> MAVDSAMELLFLDTFKHPSAEQSSHIDVVRFPCVVYINEVRVIPPGVRAHSSLPDNRAYGETSPHTFQLDLFFNNVSKPSAPVFDRLGSLEYDENTSIIFRPNSKVNTDGLVLRGWYNCLTLAIYGSVDRVISHDRDSPPPPPPPPPPPQPQPSLKRNPKHADGEKEDQFNGSPPRPQPRGPRTPPGPPPPDDDEDDPVPLPVSGDKEEDAPHREDYFEPISPDRNSVPQEGQYSDEGEVEEEQQEEGEEDEDDVDVEEEEDEDEDDRRTVDSIPEEEEEDEEEEGEEDEEGEGDDGYEQISSDEDGIADLERETFKYPNFDVEYTAEDLASVPPMTYDPYDRELVPLLYFSCPYKTTFEIEISRMKDQGPDKENSGAIEASVKLTELLDLYREDRGAKWVTALEEIPSLIIKGLSYLQLKNTKQDSLGQLVDWTMQALNLQVALRQPIALNVRQLKAGTKLVSSLAECGAQGVTGLLQAGVISGLFELLFADHVSSSLKLNAFKALDSVISMTEGMEAFLRGRQNEKSGYQKLLELILLDQTVRVVTAGSAILQKCHFYEVLSEIKRLGDHLAEKTSSLPNHSEPDHDTDAGLERTNPEYENEVEASMDMDLLESSNISEGEIERLINLLEEVFHLMETAPHTMIQQPVKSFPTMARITGPPERDDPYPVLFRYLHSHHFLELVTLLLSIPVTSAHPGVLQATKDVLKFLAQSQKGLLFFMSEYEATNLLIRALCHFYDQDEEEGLQSDGVIDDAFALWLQDSTQTLQCITELFSHFQRCTASEETDHSDLLGTLHNLYLITFNPVGRSAVGHVFSLEKNLQSLITLMEYYSKEALGDSKSKKSVAYNYACILILVVVQSSSDVQMLEQHAASLLKLCKADENNAKLQELG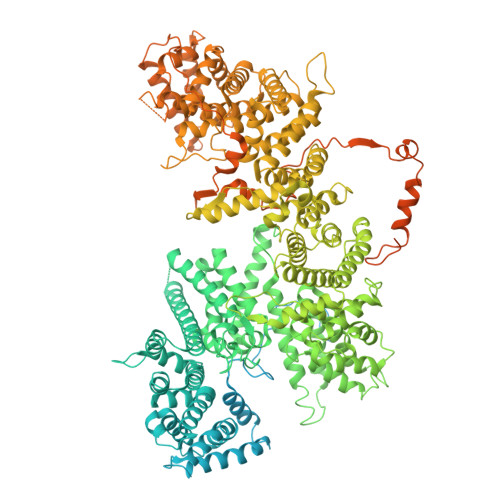KWLEPLKNLRFEINCIPNLIEYVKQNIDNLMTPEGVGLTTALRVLCNVACPPPPVEGQQKDLKWNLAVIQLFSAEGMDTFIRVLQKLNSILTQPWRLHVNMGTTLHRVTTISMARCTLTLLKTMLTELLRGGSFEFKDMRVPSALVTLHMLLCSIPLSGRLDSDEQKIQNDIIDILLTFTQGVNEKLTISEETLANNTWSLMLKEVLSSILKVPEGFFSGLILLSELLPLPLPMQTTQVIEPHDISVALNTRKLWSMHLHVQAKLLQEIVRSFSGTTCQPIQHMLRRICVQLCDLASPTALLIMRTVLDLIVEDLQSTSEDKEKQYTSQTTRLLALLDALASHKACKLAILHLINGTIKGDERYAEIFQDLLALVRSPGDSVIRQQCVEYVTSILQSLCDQDIALILPSSSEGSISELEQLSNSLPNKELMTSICDCLLATLANSESSYNCLLTCVRTMMFLAEHDYGLFHLKSSLRKNSSALHSLLKRVVSTFSKDTGELASSFLEFMRQILNSDTIGCCGDDNGLMEVEGAHTSRTMSINAAELKQLLQSKEESPENLFLELEKLVLEHSKDDDNLDSLLDSVVGLKQMLESSGDPLPLSDQDVEPVLSAPESLQNLFNNRTAYVLADVMDDQLKSMWFTPFQAEEIDTDLDLVKVDLIELSEKCCSDFDLHSELERSFLSEPSSPGRTKTTKGFKLGKHKHETFITSSGKSEYIEPAKRAHVVPPPRGRGRGGFGQGIRPHDIFRQRKQNTSRPPSMHVDDFVAAESKEVVPQDGIPPPKRPLKVSQKISSRGGFSGNRGGRGAFHSQNRFFTPPASKGNYSRREGTRGSSWSAQNTPRGNYNESRGGQSNFNRGPLPPLRPLSSTGYRPSPRDRASRGRGGLGPSWASANSGSGGSRGKFVSGGSGRGRHVRSFTR>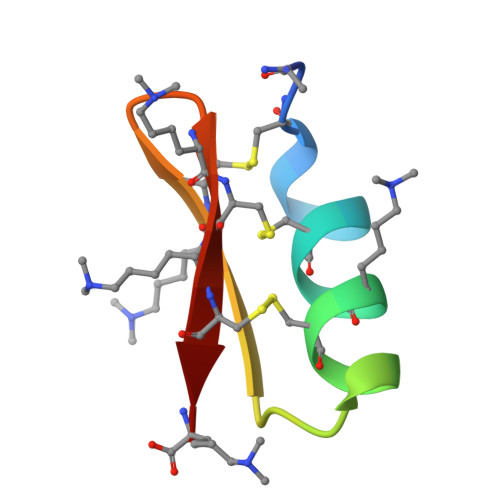[2x]AACYSSDCRVKCVAMGFSSGKCINSKCKCYK> GIDPF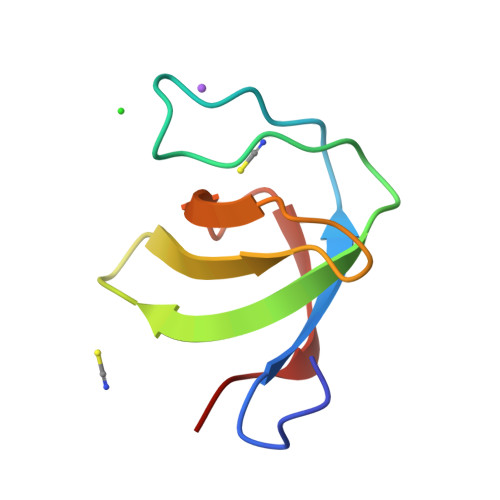TGEAIAKFNFNGDTQVEMSFRKGERITLLRQVDENWYEGRIPGTSRQGIFPITYVDVIKRPL> GPGSEFRRRRRCQVAFSYLPQNDDELELKVGDIIEVVGEVEEGWWEGVLNGKTGMFPSNFIKE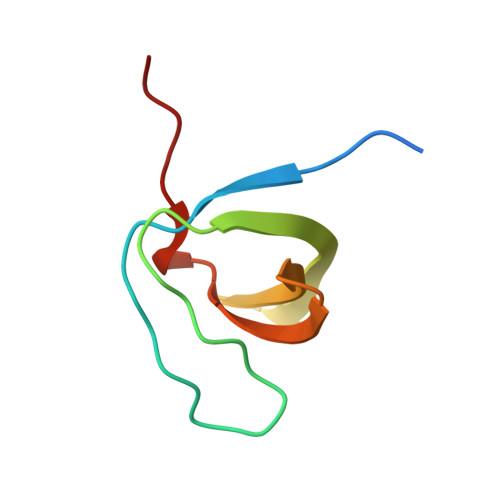LSG> MGEPAKIYINLGVQAPGPFGGGTPEEVAATLDRVKAAAPGIGIIVDLDEGSGVHRDSDHVRLYPEGAGRYTLAEEQAIVDH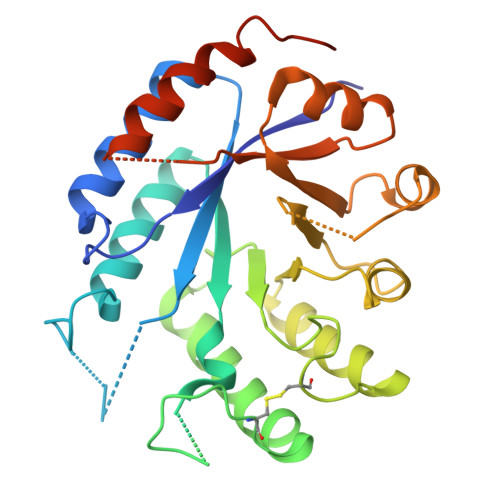AKALGAEICYHLNLTVFLPTDPVSEEERAAAKPVWTWTGLHHCIPKEKLLETLLPQKLDELEAAFPGKLDYVYLDRLFDGRCYDLTDEEVRYVLDLIKERGLGIKIESTKYLDTILESGVKVLVDEAVSEKNFDTGKAKVLDPKLFEKYPDLITVEVLYESIETIERALAAGVRNIAIHFGGYGVVSQLDEILDGVRAITENILALASAGSGHHHHHH> MNRFWNTKKFSLTNADGLCATLNEISQNDEVLVVQPSVLPVLNSLLTFQDLTQSTPVRKITLLDDQLSDDLPSALGSVPQMDLIFLIDVRTSLRLPPQLLDAAQKHNLSSLHIIYCRWKPSFQNTLEDTEQWQKDGFDLNS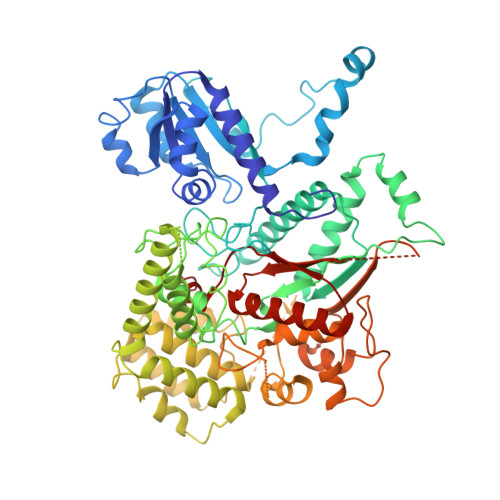KKTHFPNVIESQLKELSNEYTLYPWDLLPFPQIDENVLLTHSLYNMENVNMYYPNLRSLQSATESILVDDMVNSLQSLIFETNSIITNVVSIGNLSKRCSHLLKKRIDEHQTENDLFIKGTLYGERTNCGLEMDLIILERNTDPITPLLTQLTYAGILDDLYEFNSGIKIKEKDMNFNYKEDKIWNDLKFLNFGSIGPQLNKLAKELQTQYDTRHKAESVHEIKEFVDSLGSLQQRQAFLKNHTTLSSDVLKVVETEEYGSFNKILELELEILMGNTLNNDIEDIILELQYQYEVDQKKILRLICLLSLCKNSLREKDYEYLRTFMIDSWGIEKCFQLESLAELGFFTSKTGKTDLHITTSKSTRLQKEYRYISQWFNTVPIEDEHAADKITNENDDFSEATFAYSGVVPLTMRLVQMLYDRSILFHNYSSQQPFILSREPRVSQTEDLIEQLYGDSHAIEESIWVPGTITKKINASIKSNNRRSIDGSNGTFHAAEDIALVVFLGGVTMGEIAIMKHLQKILGKKGINKRFIIIADGLINGTRIMNSIS>[4x]MSLRVYVTGNITVDETWSIPDIPKKGASIHGVKVSQDIGGKGANQAIILSRCGIETRLIAATGNDSNGAWIRQQIKNEPLMLLPDGHFNQHSDTSIILNSADGDNAIITTTAAADTFSLDEMIPHMADAVAGDILLQQGNFSLDKTRALFQYARSRGMTTVFNPSPVNPDFCHLWPLIDIAVVNESEAELLQPYGVKTLVITQGAAGAWLVQEGQRQFCPAVPAEALDT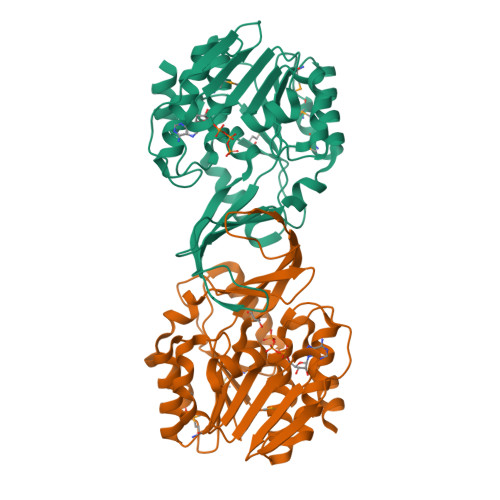TGAGDTFLAVMLASALLRGVAPDALALAHASRAAAITVSRRGTLSAFPGSRELAALLTTDGAEGHHHHHH> ANAFLEELRPGSLERECKEEQCSFEEAREIFKDAERTKLFWISYSDGDQCASSPCQNGGSCKDQLQSYICFCLPAFEGRNCETHKDDQLICVNENGGCEQYCSDHTGTKRSCRCHEGYSLLADGVSCTPTVEYPCGKIP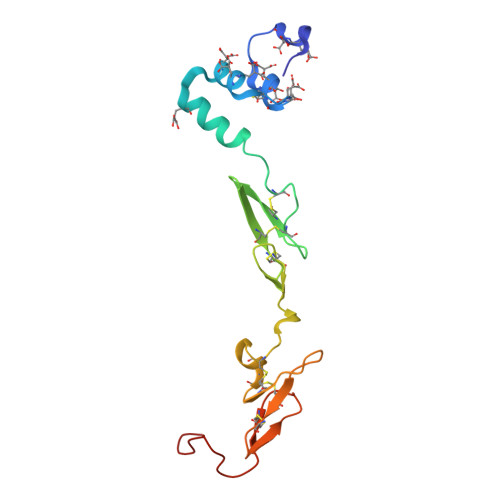ILE URIDYLYL-2'-5'-PHOSPHO-ADENOSINE | C19 H24 N7 O12 P | 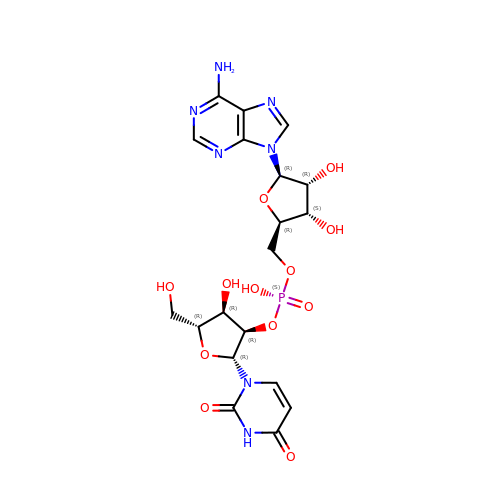QARCCHXXGAIRFS-KPKSGTNCSA-N>LSPADALRVAEDHFLRHMPDARDFADVAKYLVAKGNLHLAAFNLHQAVETAYNCYLLTLTNYSPASHNMKFLRGLSEGRDRRLIDIWPRDRQRFTTWYNIMNEAYVKARYSKRFEVSEEALTWLQERTAELHKLVETLCREHIEKLEHAAGQAANSSD[2x]

Two additional proteins, among others, are also required for Agrobacterium tumorigenesis: VirD4-coupling protein (CP) and VirD2-binding protein (VBP). VBP is responsible for recruiting VirD2–T-DNA to VirD4 CP to help localize T-DNA to the Type IV Secretion System apparatus for transfer. Sequence-based predictions revealed that VBP has two domains: an NT_KNTase -like domain at the N-terminus and a HEPN (higher eukaryotes and prokaryotes nucleotide-binding) domain at the C-terminus. We show that the C-terminal domain is the dimerization domain of VBP and only dimeric VBP is functional and essential for the induction of tumor in plants.

Subsequently, we generated a new construct that consisted of the C-terminal domain, and obtained crystals that diffracted up to 2.7 Å resolution. The structure was determined using the single wavelength anomalous diffraction (SAD) method.The asymmetric unit consists of two monomers forming a tight dimer. Each monomer contains a six-helix bundle with three long anti-parallel α helices (α1, α2, and α6) that forms the major part of this domain, and three shorter helices (α3, α4 and α5) that stack at an angle to the long helices. The monomers are arranged as anti-parallel dimers with a large buried surface area of 1203 Å2 (or 14% of the total surface area of each monomer). The dimer is held together by tight interactions between α1 and α2 helices from both monomers. A DALI search for the structural homologs of VBP C-terminal domain identified several proteins with a HEPN domain; this confirmed that the C-terminal domain of VBP adopts a HEPN fold (hereafter referred to as HEPN domain). The structural analysis indicated that the HEPN dimer is held together by contacts throughout helices α1 and α2; in particular, residues Asp173, Lys184 and Asn186 of the HEPN domain play important roles in maintaining the dimer. Asn186 is located at the edge of a loop connecting the α1 and α2 helices of the dimer interface. This residue, along with Lys184 and Asp173 of one monomer, is involved in hydrogen bonding contacts with Asp173 and Asn186, Lys184 of the second monomer. We found that a single substitution of Asp173Asn, Lys184Asp or Asn186Asp in the HEPN domain is sufficient to disrupt dimer formation, as verified by size-exclusion chromatography and analytical ultracentrifugation experiments. The structural similarity observed between the HEPN domain of VBP and kanamycin nucleotidyltransferase, as well as the results from our ITC experiments, suggest that a nucleotide binding pocket is formed by the dimeric interface in this protein.>MRSRRVDVMDVMNRLILAMDLMNRDDALRVTGEVREYIDTVKIGYPLVLSEGMDIIAEFRKRFGCRIIADFKVADIPETNEKICRATFKAGADAIIVHGFPGADSVRACLNVAEEMGREVFLLTEMSHPGAEMFIQGAADEIARMGVDLGVKNYVGPSTRPERLSRLREIIGQDSFLISPGVGAAGGDPGETLRFADAIIVGASIYLADNPA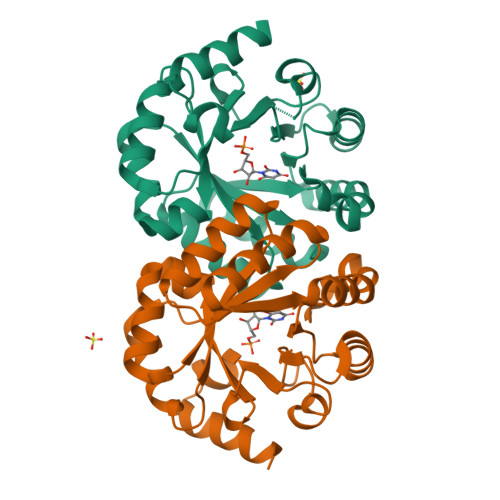AAAAGIIESIKDLLNP[2x]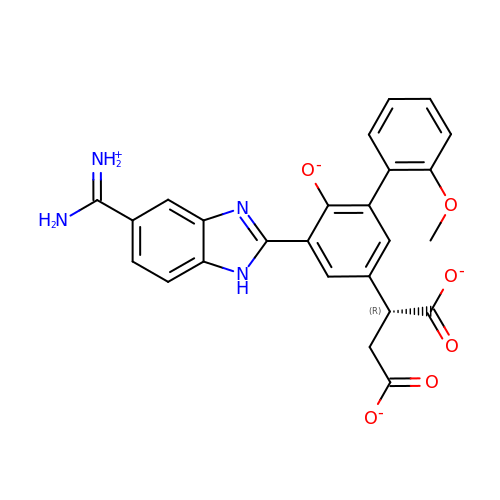2-(5-{5-[AMINO(IMINIO)METHYL]-1H-BENZIMIDAZOL-2-YL}-2'-METHOXY-6-OXIDO-1,1'-BIPHENYL-3-YL)SUCCINATE | C25 H20 N4 O6 | HVNXYZZCSQONQC-OAHLLOKOSA-L> GSTGSPPGPPTSIHVEEITDTTATLSWRPGPDNHSPITAYTIQARTPFSLGWQAVSTVPEVVGGSHLTATVIELNPWVEYEFRVLASNAVGTGEPSKPSKKARTKDTVPKVTPANVSGGGGSRSELVITWEPVPEELQNGAGFGYVVAFRPFGSTGWMQAAVPSPEASKYVFKNETILPFSPFQVKVGAYNNKGEGPFGPVITIYSAEEEPGRAPSRLRAKSLSASDVEVSWKALPWSTSKKRVLGYELRYWEKNEKEDASSVLRTVGNRTLAIIQGLKGSSTYYITVRAYNTAGTGPPSPVVNITTKK;> GPGSIEVPSDDSVGLLAEPQVAMFCGKLNMHINVQSGKWEPDPTGTKSCISTKEGILKYCQEVYPDLQITNVVEANQPVSIQNWCKMGRRQCRSHTHIVVPYRCLVGEFVSDALLVPDKCKFLHQERMDMCESHLHWHTVAKESCGDRSMNLHDYGMLLPCGIDRF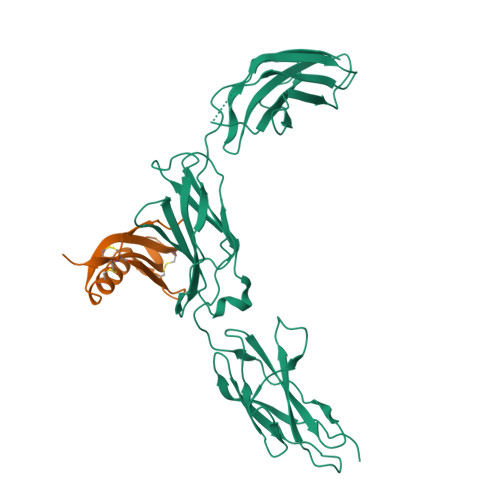RGVEFVCCPMEEQKDLDSEAAA> LPRETDEEPEEPGKKGSFVEMVDNLRGKSGQGYYVEMTVGSPPQTLNILVDTGSSNFAVGAAPHPFLHRYYQRQLSSTYRDLRKGVYVPYTQGKWEGELGTDLVSIPHGPNVTVRANIAAITESDKFFINGSNWEGILGLAYAEIARPDDSLEPFFDSLVKQTHVPNLFSLQLCGAGFPLNQSEVLASVGGSMIIGGIDHSLYTGSLWYTPIRREWYYEVIIVRVEINGQDLKMDCKEYNYDKSIVDSGTTNLRLPKKVFEAAVKSIKAASSTEKFPDGFWLGEQLVCWQAGTTPWNIFPVISLYLMGEVTNQSFRITILPQQYLRPVEDVATSQDDCYK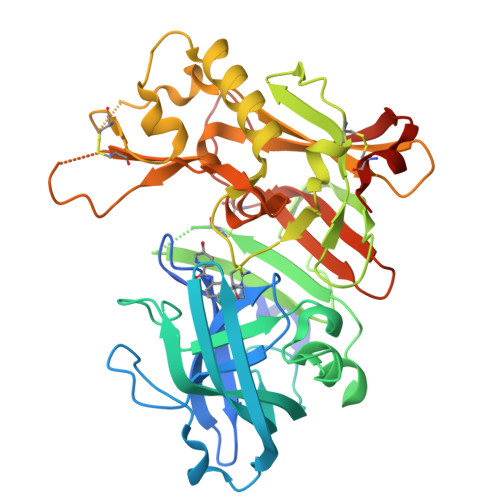FAISQSSTGTVMGAVIMEGFYVVFDRARKRIGFAVSACHVHDEFRTAAVEGPFVTLDMEDCGYNIPQTDEST> GDIKPLYCVPASMTLLFQESGHKKGSFLEGSEVRTIVINYAKKNDLVDADNKNLVRLDPILCDCILEKNEQHTVMKLPWDSLLTRCLEKLQPAYQVTLPGQEPIVKKGRICPIDITLAQRASNKKVTVVRNLEAYGLDPYSVAAILQQRCQASTTV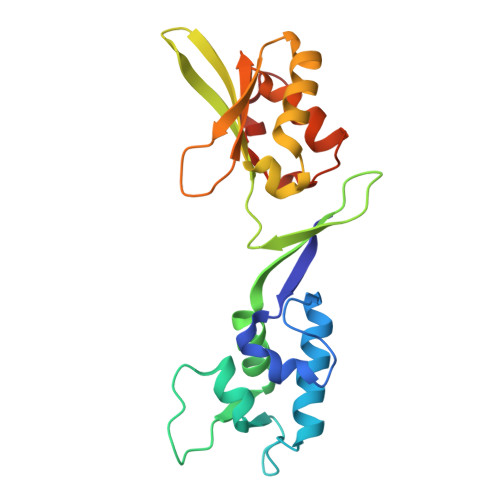NPAPGAKDSLQVQIQGNQVHHLGWLLLEEYQLPRKHIQGLEKALKPGKKK>MSEPMMWLLVRGVWETLAMTFVSGFFGFVIGLPVGVLLYVTRPGQIIANAKLYRTVSAIVNIFRSIPFIILLVWMIPFTRVIVGTSIGLQAAIVPLTVGAAPFIARMVENALLEIPTGLIEASRAMGAT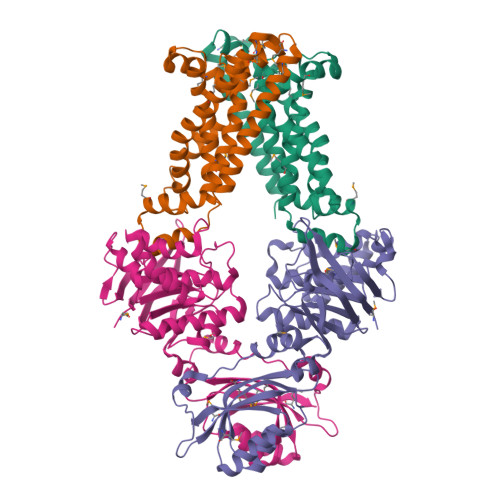PMQIVRKVLLPEALPGLVNAATITLITLVGYSAMGGAVGAGGLGQIGYQYGYIGYNATVMNTVLVLLVILVYLIQFAGDRIVRAVTRK[2x];>[2x]MGHHHHHHHHHHSSGHIDDDDKHMIKLSNITKVFHQGTRTIQALNNVSLHVPAGQIYGVIGASGAGKSTLIRCVNLLERPTEGSVLVDGQELTTLSESELTKARRQIGMIFQHFNLLSSRTVFGNVALPLELDNTPKDEVKRRVTELLSLVGLGDKHDSYPSNLSGGQKQRVAIARALASNPKVLLCDQATSALDPATTRSILELLKDINRRLGLTILLITHEMDVVKRICDCVAVISNGELIEQDTVSEVFSHPKTPLAQKFIQSTLHLDIPEDYQERLQAEPFTDCVPMLRLEFTGQSVDAPLLSETARRFNVNNNIISAQMDYAGGVKFGIMLTEMHGTQQDTQAAIAWLQEHHVKVEVLGYV> MIRNFHSLVKRVPRLALTPFFGFRTSMTLADKKLSTGEASVVLAEKIKGITQQNDITEYGTVISIGDGIARVFGLTKVQAGEMVEFKSGIRGMALNLETDNVGVVVLGNDRDIKEGDVVKRTGAIVDVPIGEAMCGRVFDALGNPIDGLGPLKTTQRARVEIKAPGIIPRQSVRQPMQTGIKCVDSLVPIGRGQRELIIGDRQTGKTAIAIDTILNQKEAFNTGDVKKQLYCIYVAVGQKRSTIANLVSILKQHDCMK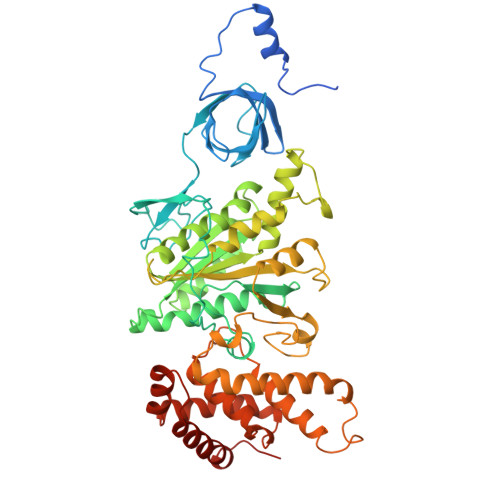FTIVVCATASDAAPLQFLAPYSGCAIGEFFRDNGKHALIIYDDLSKQAVAYRQMSLLLRRPPGREAYPGDVFYLHSRLLERAAKMNDSLGGGSLTALPVIETQAGDVSAYIPTNVISITDGQIFLETELFYKGIRPAINVGLSVSRVGSAAQIKAMKKIAGNLKLTLATYRELAAFSQFGSDLDAKTQQQLNTGERLVEMLKQNQYTPMKVEEQVCIIFAGVKGFLDALVTSEVLKFEKKFLEHVRTNHSALLKRIRDSGDLSEVDTNELNTIIPLFIQEGGFKLKAQ> TSSINFLTSDDDASAAAMEAFIGTNHHSSLFPPPPQQPPQP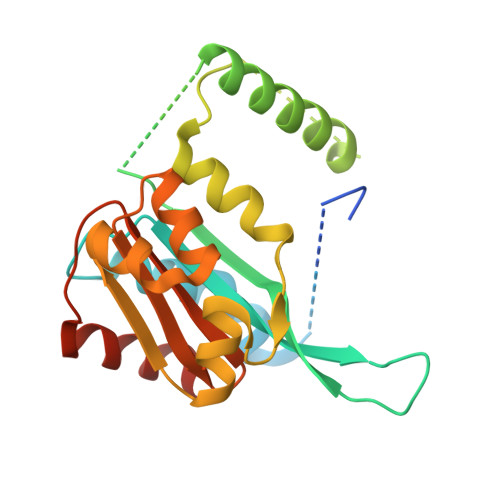QFNEDTLQQRLQALIESAGENWTYAIFWQISHDFDSSTGDNTVILGWGDGYYKGEEDKEKKKNNTNTAEQEHRKRVIRELNSLISGGIGVSDESNDEEVTDTEWFFLVSMTQSFVNGVGLPGESFLNSRVIWLSGSGALTGSGCERAGQGQIYGLKTMVCIATQNGVVELGSSEVISQSSDLMHKVNNLFNFNNGGG N~3~-(tetrahydro-2H-pyran-4-yl)-N~6~-[5-(tetrahydro-2H-pyran-4-ylmethyl)[1,2,4]triazolo[1,5-a]pyridin-2-yl]-1H-indazole-3,6-diamine 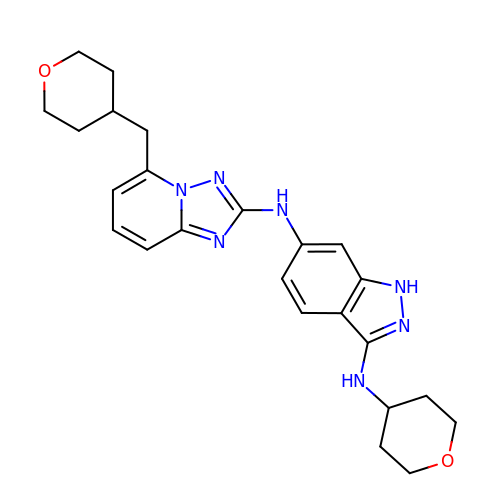| C24 H29 N7 O2 | SHDAHIVOLRESPS-UHFFFAOYSA-N> MRRRIPSRTPGSGAKQKSWFPRRSLQVLLSAGMLSGLLGTPAALAAEPAPLPA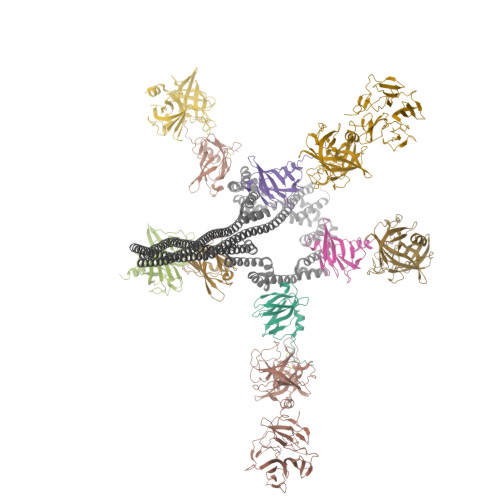NVRADIVGYWETGGAGLKAAAEQALLGGDEAIRKFLADAPSIQHDDNRIDAARMAMTGGSGLRQAAKDAIRLSPAELEKFLLYGYEEPLDDDHKVEIARLINLGGPGVREAGKAALQGTAEERELFLNSGQYTAQQDDNRVDVARLATTGGPNVQAAAKVALRGTPEDMVEFLEVGQFTARNRDQEHATIAELIKQAELAGKQADDARKTAEESSKKAVDASQLAKEAAQKAAEETEAAKDDSQKAAVKAKQAADAARAAADAAQEAIGSANAANRAARRAALAAAQTASAATAAAEAANKAYKAAIAAAGDEGKADEAKEAAKQARAAADAATKSGLAAENAGLASAAAATASTAAKSASSNARAAAGAAEEANQHADAAGVHSNEAALAAAEARRHADAADRAADRSSALAQRAATAAYGARDAANSAAEHANKAADYADESAAHAGDSAAYAATAKRNAQAAQEAAKTATAAVTKANEIFKLARETETANLETRTDAAIERARSMKSASETSITASATTQVEALALNDTATELAKEASRPDIDVQATAAKGRQLAMQAMKLLGPWHQEAAARALSGTDQDVLDYLRTRWKEANHNDIRQQIVDLSTQSPYASVRTAAAEALNGTPEQIEAFHTTGQYTAGSDDMKVDVARLANTGGPGVSQAAKTALADGTGKTLATFLQIGQYGERLSDEKVVTARLAETGSPEVQAAAKIALAGPPELLHEFVTTGQYMAKRKDDLADVHVNQVERLLAEGSLIAAEANEDAWRATEAAATAEGAAADAATAAEKAEASAAQAKQHAADADASADAATRSAADAAASAATARDAADRAAQDATAAENSAAEAAFSAAYARDSASKADDAADRARASALAAGKSADEAEAEAKEAWKTTRALAEKEAEEARRKAAEERKRQQEQAGEPKRVCIPHPTRETMIPIMPCAASPDDSMIMPGPVDPTIRAVVWELAGLNDIKACIDKPLSGNCVMAVVGVTPWGKFKLVSKLGNGLDAVKDARGARRTVACLTGAAHSFPAGTRVLMADGTRRSIEQIEAGDLVTATDPTTGETGARTVTRTIHTPDDRNFTDVALADGSTLTSTTHHPYWSQNDQTWKNAGDLEAGDTLRTPQNTAVVIAATHDWPGLQDAYDLTVDGFHSYYVSTGTTDVLVHNNDNPCPDWVSKAWKKLPKRKSGDPTSGYVFEADGTLVWDSVLTSGRSPLSEDISAFLKGSPDFPNFPGYADVAHHAEAKIAWEMRTKMGKGKKLHIVINTNYVCPKVSSPNSMGCKQAVPAILYEDQTLYVHYPGASDALELKGTAKR;>[5x]MANTSRTRQALMAIAVSVLAAGVTTLGVAHADNGDAVAAAAEMPQAVEDFSYPGAAKIQAETGAILKRGNGHMLMTSCDGSEDIQVMSRTGQKDFCFNVMAKPAYLTLEVPQAYGIWTSADPVKTTIKDTDGTATVINAPANDFTGYGEAGSTGEPTTLIELRVAG;>[5x]MFRMPRPIRATALSAAVLAGALASTPAQATVGDPTTDAKLDFTARLTIGTDYRSCSGALVDTQWVLTAASCFADDPNQPDTVAAGKPAQLTRATVGRADSNIANGYVREVVELVPHPERDMVLARLDKAIPDIAPVRLASDAPTAGTPLTAVGFGRTKDEWVPIQRHQGAFTVTSVTAGAVNVTGQGGDAICAGDTGGPLLQDKNGTLHLVGVNNRSMQGGCYGSETTSTDAIAAMSDADFVTQTVNRDLGTGNLSDLVASADFNSDGRTDVAAVLEDGSLHAFYAKPDGTLEYGRELWNDNTWSPMVQIIGGDFNSDGNGDIAAVRSDGTLNLYTGTATGILNKSKPMWHDTSWKTIKQVTRFKFNGRDGLVAQWGDGNLYGYYTGTDGTLTGTKVKMWPDATWGKTRLTGTADINADGRDDLTAVRDDGSLNWYAGNTKGGLDAARKLWPDNTWTPMKRIIGGDFNGDNKGDIAAVGGQSTLLLYTGTGTGTLNKGIAMRPASGSHHHHHHHH Human respiratory syncytial virus (RSV) is a nonsegmented, negative strand RNA virus (NSV) that causes lethal lower respiratory tract infections and continues to pose health threats to infants, the elderly, and people with compromised immune systems worldwide. The RSV genome encodes the nucleoprotein (N) that forms helical assembly to encapsulate and protect the RNA genome from degradation, and to serve as a template for transcription and replication. N consists of 391 amino acids with N-terminal domain (NTD) (residues 36–253) and C-terminal domain (CTD) (residues 254–360), which is one of the most abundant proteins that forms the helical assembly with viral RNAs to provide protection from degradation and to participate in transcription and replication as the template. The RSV-N protein consists of the N-terminal lobe and the C-terminal lobe linked by L14 that is conserved among all negative strand RNA viruses.

We prepared the RSV nucleocapsid assembly by recombinant expression of the full-length N in HEK293 cells. Final three-dimensional (3D) reconstruction yielded the RSV nucleocapsid of roughly one left-handed helical turn of 10 N protomers at 3.96 Å resolution, with the top view resembling the decameric ring architecture as reported in previous crystal structure. Modeling of individual N resembled the previous crystal structure with well resolved density for protein side chains and RNA bases and similar secondary structure. All nucleotides were modeled as uridine due to the random composition of cellular RNA, with each N bound to 7-nt RNA. In our nucleocapsid-like assembly structure, we observed seven nucleotides encapsulated in the overall positively charged cleft of each N protomer, with four bases facing outward and three facing inward. The positively charged residues K170, R184 and R185 in N-terminal lobe form electrostatic interactions with the phosphate backbone of the nucleotides pointing inward, whereas S313, T315 and Y337 in C-terminal lobe form hydrogen bonds with the phosphate backbone of the nucleotides pointing outward to the solvent. We observed that Y88 in β3 and D221 in α7 of N interact with R234 in L13 of N + 1 via hydrogen bond and salt bridge, validating the key role of R234 in interaction interface. In addition, we identified interactions between Q26 in L2 of N and Y38 in α2 of N + 1 through hydrogen bond as predicted by previous study. The absence of Y38 phosphorylation in our structure suggests that viral transcription and replication likely utilize less compact nucleocapsid template.

>[5x]MALSKVKLNDTLNKDQLLSSSKYTIQRSTGDSIDTPNYDVQKHINKLCGMLLITEDANHKFTGLIGMLYAMSRLGREDTIKILRDAGYHVKANGVDVTTHRQDINGKEMKFEVLTLASLTTEIQINIEIESRKSYKKMLKEMGEVAPEYRHDSPDCGMIILCIAALVITKLAAGDRSGLTAVIRRANNVLKNEMKRYKGLLPKDIANSFYEVFEKHPHFIDVFVHFGIAQSSTRGGSRVEGIFAGLFMNAYGAGQVMLRWGVLAKSVKNIMLGHASVQAEMEQVVEVYEYAQKLGGEAGFYHILNNPKASLLSLTQFPHFSSVVLGNAAGLGIMGEYRGTPRNQDLYDAAKAYAEQLKENGV>MQKVESIIIGGGPCGLSAAIEQKRKGIDTLIIEKGNVVESIYNYPTHQTFFSSSDKLSIGDVPFIVEESKPRRNQALVYYREVVKHHQLKVNAFEEVLTVKKMNNKFTITTTKDVYECRFLTIATGYYGQHNTLEVEGADLPKVFHYFKEAHPYFDQDVVIIGGKNSAIDAALELEKAGANVTVLYRGGDYSPSIKPWILPN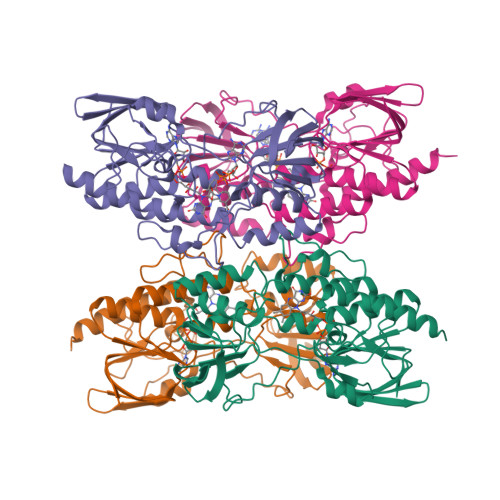FTALVNHEKIDMEFNANVTQITEDTVTYEVNGESKTIHNDYVFAMIGYHPDYEFLKSVGIQINTNEFGTAPMYNKETYETNIENCYIAGVIAAGNDANTIFIENGKFHGGIIAQSMLAKKQTPLES[8x]> SNAMLSGKARAHTNIALIKYWGKANEEYILPMNSSLSLTLDAFYTETTVTFDAHYSEDVFILNGILQNEKQTKKVKEFLNLVRQQADCTWFAKVESQNFVPTAAGLASSASGLAALAGACNVALGLNLSAKDLSRLARRGSGSACRSIFGGFAQWNKGHSDETSF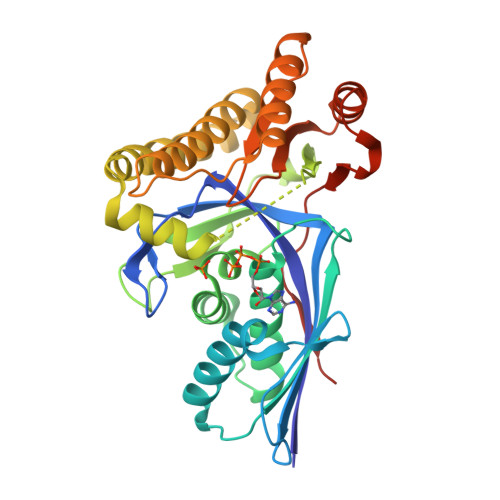AENIPANNWENELAMLFILINDGEKDVSSRDGMKRTVETSSFYQGWLDNVEKDLSQVHEAIKTKDFPRLGEIIEANGLRMHGTTLGAVPPFTYWSPGSLQAMALVRQARAKGIPCYFTMDAGPNVKVLVEKKNLEALKTFLSEHFSKEQLVPAFAGPGIELFETKGMDK> MNTPEHMTAVVQRYVAALNAGDLDGIVALFADDATVEDPVGSEPRSGTAAIREFYANSLKLPLAVELTQEVRAVANEAAFAFIVSFEYQGRKTVVAPIDHFRFNGAGKVVSMRALFGEK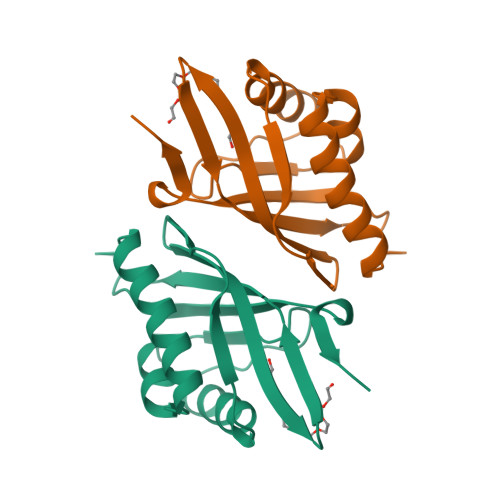NIHAGA> GPYYPTNKLQAAVMETDRENAIIRQRNDEIPTRTLDTAIFTDASTVASAQIHLYYNSNIGKIIMSLNGKKHTFNLYDDNDIRTLLP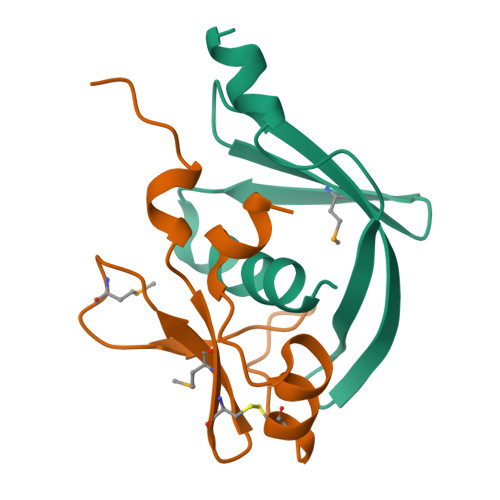ILLLSK;> GPNMFFMPKRKIPDPIDRLRRANLACEDDKLMIYGLPWMTTQTSALSINSKPIVYKDCAKLLRSINGSQPVSLNDVLRR> QPVTGGAEALRIRWSKAPCRFCGTGCGVMVGTRDGQVVATHGDTQAEVNRGLNCVKGYFLSKIMYGEDRLTTPLLRMKDGVYHKEGEFAPVSWDEAFDVMAAQAKLVL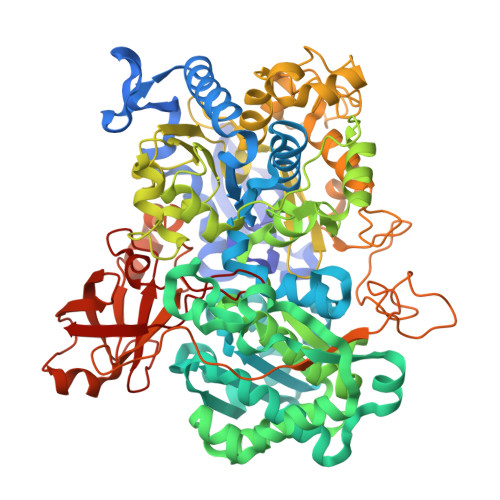KEKAPEAVGMFGSGQWTIWEGYAASKLMRAGFRSNNLDPNARHCMASAATAFMRTFGMDEPMGCYDDFEAADAFVLWGSNMAEMHPILWSRLTDRRLSHEHVRVAVLSTFTHRSSDLSDTPIIFRPGTDRAILNYIAHHIISTGRVNRDFVDRHTNFALGATDIGYGLRPEHQLQLAAKGAADAGAMTPTDFETFAALVSEYTLEKAAEISGVEPALLEELAELYADPDRKWMSLWTMGFNQHVRGVWANHMVYNLHLLTGKISEPGNSPFSLTGQPFACGTAREVGTFAHRLPADMVVTNPEHRAHAEEIWKLPAGLLPDWVGAHAVEQDRKLHDGEINFYWVQVNNNMQAAPNIDQETYPGYRNPENFIVVSDAYPTVTGRAADLVLPAAMWVEKEGAYGNAERRTHFWHQLVEAPGEARSDLWQLMEFSKRFTTDEVWPEEILSAAPAYRGKTLFEVLFANGSVDRFPASDVNPDHANHEAALFGFYPQKGLFEEYAAFGRGHGHDLAPFDTYHEVRGLHWPVVEGEETRWRYREGFDPYVKPGEGLRFYGKPDGRAVILGVPYEPPAESPDEEFGFWLVTGRVLEHWHSGSMTLRWPELYKAFPGAVCFMHPEDARSRGLNRGSEVRVISRRGEIRTRLETRGRNRMPRGVVFVPWFDASQLINKVTLDANDPISRQTDFKKCAVKIEAV> MIHELLLALSGYPGSIFTWNKRSGLQVSQDFPFLHPSETSVLNRLCRLGTDYIRFTEFIEQYTGHVQQQDHHPSQQGQGGLHGIYLRAFCTGLDSV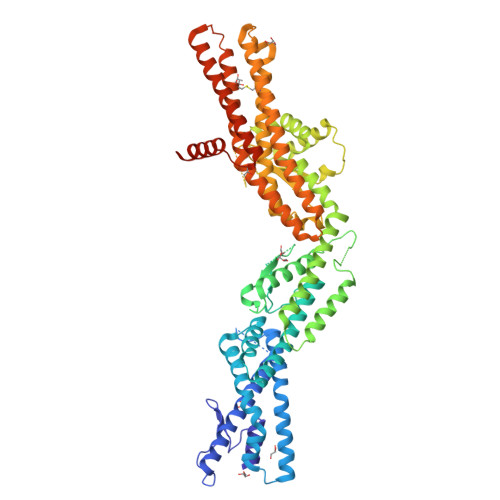LQPYRQALLDLEQEFLGDPHLSISHVNYFLDQFQLLFPSVMVVVEQIKSQKIHGCQILETVYKHSCGGLPPVRSALEKILAVCHGVMYKQLSAWMLHGLLLDQHEEFFIKQGPSSGNVSAQPEEDEEDLGIGGLTGKQLRELQDLRLIEEENMLAPSLKQFSLRVEILPSYIPVRVAEKILFVGESVQMFENQNVNLTRKGSILKNQEDTFAAELHRLKQQPLFSLVDFEQVVDRIRSTVAEHLWKLMVEESDLLGQLKIIKDFYLLGRGELFQAFIDTAQHMLKTPPTAVTEHDVNVAFQQSAHKVLLDDDNLLPLLHLTIEYHGKEHKDATQAREGPSRETSPREAPASGWAALGLSYKVQWPLHILFTPAVLEKYNVVFKYLLSVRRVQAELQHCWALQMQRKHLKSNQTDAIKWRLRNHMAFLVDNLQYYLQVDVLESQFSQLLHQINSTRDFESIRLAHDHFLSNLLAQSFILLKPVFHCLNEILDLCHSFCSLVSQNLGPLDERGAAQLSILVKGFSRQSSLLFKILSSVRNHQINSDLAQLLLRLDYNKYYTQAGGTLGSFGMCGRLEHHHHHH> MPDYSYRPTIGRTYV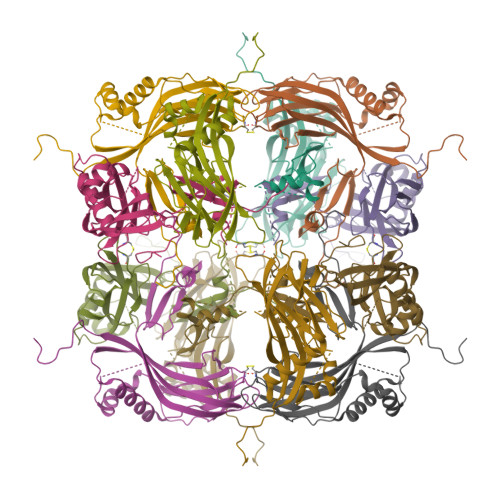YDNKYYKNLDAVIKNAKRKKHFAEHEIEEATLDPLDNYLVAEDPFLGPGKNQKLTLFKEIRNVKPDTMKLVVGWKGKEFYRETWTRFMEDSFPIVNDQEVMDVFLVVNMRPTRPNRCYKFLAQHALRCDPDYVPHDVIRIVEPSWVGSNNEYRISLAKKGGGCPIMNLHSEYTNSFEQFIDRVIWENFYKPIVYIGTDSAEEEEILLEVSLVFKVKEFAPDAPLFTGPAY dibenzothiophene 5-oxide | C12 H8 O S | 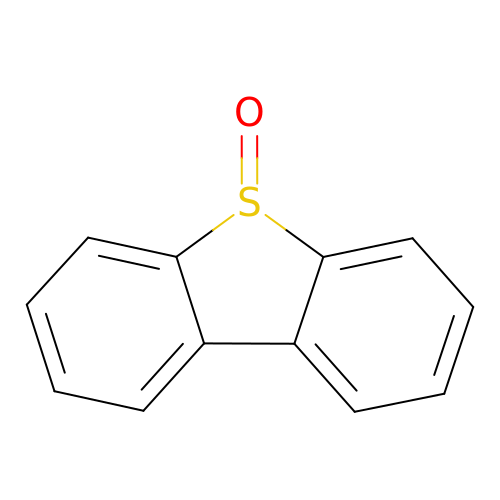NGDPCAMPVQYGCW-UHFFFAOYSA-N In the present work, we identified deoxycytidine kinase (dCK) as the target responsible for the sensitisation of various cancer cell lines to gemcitabine, using reverse-proteomics. dCK is a key enzyme in the nucleoside salvage pathway and recycles bases and nucleosides originating from the degradation of RNA and DNA to achieve the biosynthesis of deoxyribonucleotides, which are required for DNA replication and repair. This cytosolic nucleoside kinase catalyses the 5′-phosphorylation of 2′-deoxycytosine (2′dC), 2′-deoxyadenosine (2′dA) and 2′-deoxyguanosine (2′dG). dCK is also responsible for the initial phosphorylation of numerous anticancer and antiviral nucleoside analogues. dCK adds the first phosphoryl group to nucleosides analogues and is usually the rate-limiting enzyme of the overall process of converting nucleosides to their deoxynucleoside triphosphate form. Hence, dCK is clinically important because of its relationship to both drug resistance and sensitivity. Previous work has revealed that dCK can adopt several distinct conformations, which are a function of the nature of the nucleoside and nucleotide bound.

In order to understand this activation mechanism, we solved crystal structures of dCK in complex with masitinib/UDP and imatinib/UDP. We found that the masitinib pyridine ring mimics a pyrimidine base in the nucleoside binding site, while the rest of the molecule extends to a cavity only available in the ‘open’ conformation of dCK. The binding mode of imatinib was similar to the one observed for masitinib; however, the pyridine ring in this case was slightly displaced from the nucleoside binding site, as the angle of the pyrimidine moiety (meta) prevents the pyridine ring reaching the bottom of the cavity and the pyridine ring extends to the sugar moiety cavity. This structural observation could explain the less pronounced potentiation effect on dCK enzymatic activity of imatinib vs. masitinib. For both molecules, interactions with dCK mainly involve non-polar interactions, without direct polar interactions. Additionally, for each ligand-bound structure, a supplementary electron density was present at the top of the cavity, likely corresponding to a second molecule of compound interacting weakly with the first one in a similar binding mode as the ‘F-series’ inhibitors reported previously. Moreover, it should be noted that masitinib and imatinib were able to open dCK in situ, since we were able to obtain these 3D structures in the ‘open’ conformation by soaking the protein kinase inhibitors in a ‘closed’ dCK crystal. The binding of these compounds also released the monophosphorylated substrate (2′-deoxycytidine-5′-monophosphate), observed in the ‘closed’ dCK crystal and still present in the other nucleoside binding site subunit, elucidating at the same time its mechanism of action.

>[4x]MSYYHHHHHHLESTSLYKKAGLENLYFQGMATPPKRSSPSFSASSEGTRIKKISIEGNIAAGKSTFVNILKQLSEDWEVVPEPVARWSNVQSTQDEFEELTMSQKNGGNVLQMMYEKPERWSFTFQTYACLSRIRAQLASLNGKLKDAEKPVLFFERSVYSDRYIFASNLYESECMNETEWTIYQDWHDWMNNQFGQSLELDGIIYLQATPETCLHRIYLRGRNEEQGIPLEYLEKLHYKHESWLLHRTLKTNFDYLQEVPILTLDVNEDFKDKYESLVEKVKEFLSTL>[2x]MTSCHIAEEHIQKVAI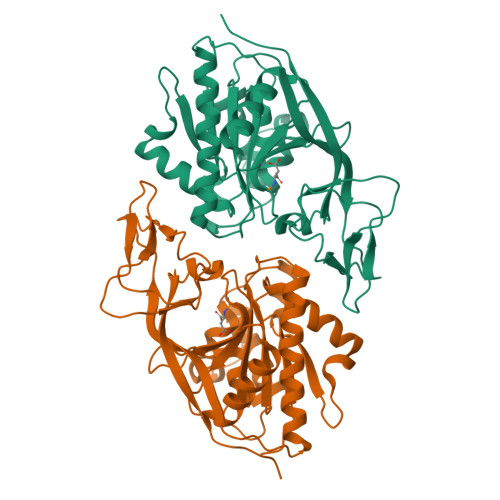FGGTHGNELTGVFLVKHWLENGAEIQRTGLEVKPFITNPRAVKKCTRYIDCDLNRIFDLENLGKKMSEDLPYEVRRAQEINHLFGPKDSEDSYDIIFDLHNTTSNMGCTLILEDSRNNFLIQMFHYIKTSLAPLPCYVYLIEHPSLKYATTRSIAKYPVGIEVGPQPQGVLRADILDQMRKMIKHALDFIHHFNEGKEFPPCAIEVYKIIEKVDYPRDENGEIAAIIHPNLQDQDWKPLHPGDPMFLTLDGKTIPLGGDCTVYPVFVNEAAYYEKKEASAKTTKLTLNAKSIRCCLH>MSAKKIVLKSSDGESFEVEEAVALESQTIAHMVEDDCVDNGVPLPNVTSKILAKVIEYCKRHVEAAASKAEAVEGAATSDDDLKAWDADFMKIDQATLFELILAANYLNIKNLLDLTCQTVADMIKGKTPEEIRTTFNIKNDFTPEEEEEVRRENQWAFE[8x];>[8x]MEDPDIKRCKLSCVATVDDVIEQVMTYITDPKDRDSASLVCRRWFKIDSETREHVTMALCYTATPDRLSRRFPNLRSLKLKGKPRAAMFNLIPENWGGYVTPWVTEISNNLRQLKSVHFRRMIVSDLDLDRLAKARADDLETLKLDKCSGFTTDGLLSIVTHCRKIKTLLMEESSFSEKDGKWLHELAQHNTSLEVLNFYMTEFAKISPKDLETIARNCRSLVSVKVGDFEILELVGFFKAAANLEEFCGGSLNEDIGMPEKYMNLVFPRKLCRLGLSYMGPNEMPILFPFAAQIRKLDLLYALLETEDHCTLIQKCPNLEVLETRNVIGDRGLEVLAQYCKQLKRLRIERGADEQGMEDEEGLVSQRGLIALAQGCQELEYMAVYVSDITNESLESIGTYLKNLCDFRLVLLDREERITDLPLDNGVRSLLIGCKKLRRFAFYLRQGGLTDLGLSYIGQYSPNVRWMLLGYVGESDEGLMEFSRGCPNLQKLEMRGCCFSERAIAAAVTKLPSLRYLWVQGYRASMTGQDLMQMARPYWNIELIPSRRVPEVNQ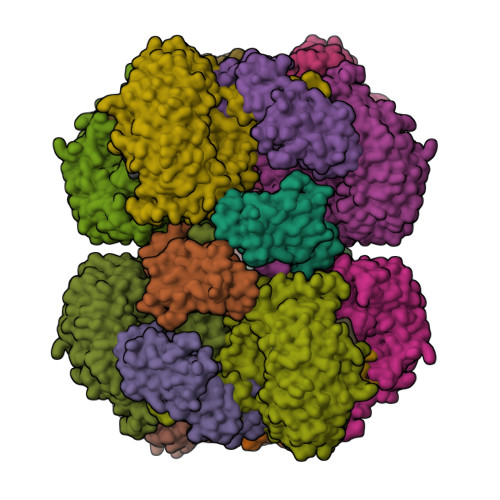QGEIREMEHPAHILAYYSLAGQRTDCPTTVRVLKEPI;>RRASLHRFLEKRKDRVTSKAPY[7x]>[12x]MERKISRIHLVSEPSITHFLQVSWEKTLESGFVITLTDGHSAWTGTVSESEISQEADDMAMEKGKYVGELRKALLSGAGPADVYTFNFSKESCYFFFEKNLKDVSFR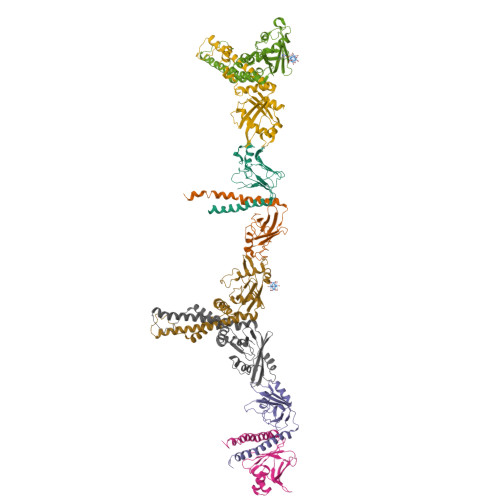LGSFNLEKVENPAEVIRELICYCLDTIAENQAKNEHLQKENERLLRDWNDHHHHHH;>[12x]MEELEQGLLMQPWAWLQLAENSLLAKVFITKQGYALLVSDLQQVWHEQVDTSVVSQRAKELNKRLTAPPAAFLCHLDNLLRPLLKDAAHPSEATFSCDCVADALILRVRSELSGLPFYWNFHCMLASPSLVSQHLIRPLMGMSLALQCQVRELATLLHMKDLEIQDYQESGATLIRDRLKTEPFEENSFLEQFMIEKLPEACSIGDGKPFVMNLQDLYMAVTTQHHHHHH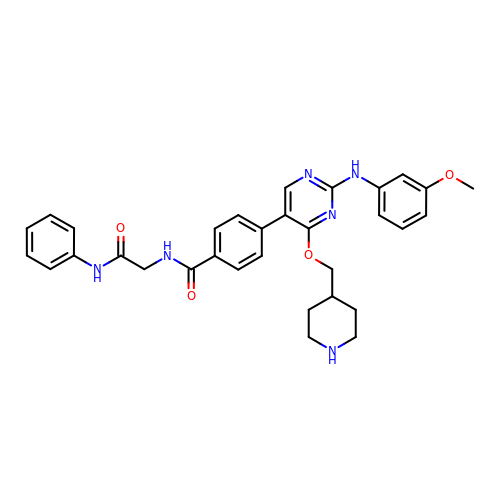4-{2-[(3-methoxyphenyl)amino]-4-[(piperidin-4-yl)methoxy]pyrimidin-5-yl}-N-[2-oxo-2-(phenylamino)ethyl]benzamide | C32 H34 N6 O4 | AJPBKLULISUYTP-UHFFFAOYSA-N2-ethylpyridine-4-carboximidothioic acid | C8 H10 N2 S | 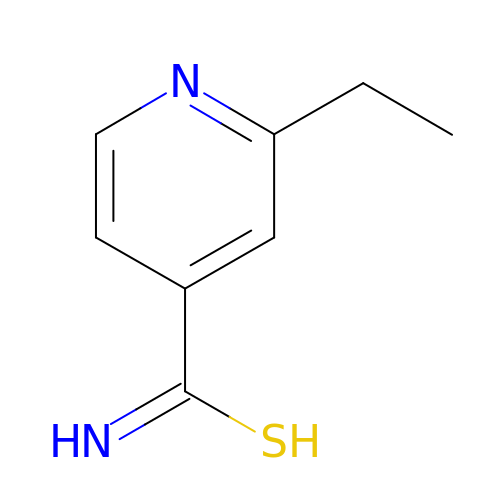AEOCXXJPGCBFJA-UHFFFAOYSA-N>[2x]MHHHHHHITSLYKKAGFMRKNFL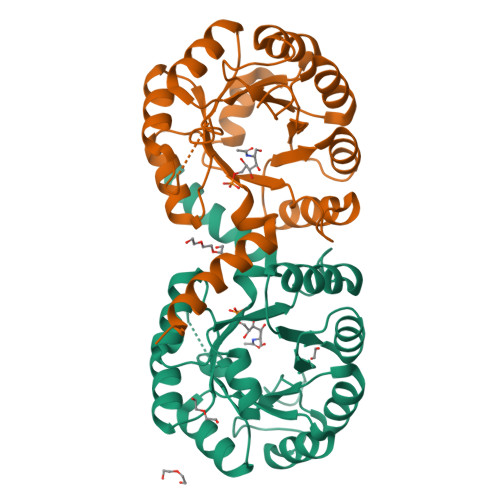NIEELKRFLNGQTVVSIQPVTGSPLDKTDFIVAMAIAVEQAGAKALRIEGVSNVAAVSAAVTIPIIGIVKRDLPDSPVRITPFVSDVDGLANAGATVIAFDATNRTRPESRERIAQAIKNTGCFAMADCSTFEDGLWANSQGVEIVGSTLSGYVGDIEPTVPDFQLVKAFSEAGFFTMAEGRYNTPELAAKAIESGAVAVTVGSALTRLEVVTQWFNNATQAAGERKCAH>[2x]GSVYLRYFKGLILSDAYAPGLKWSDELKAYSALAFKYRDVRKYFLEKEIEVEENVIDSLPFPLIKDKIELRDYQAEAVKAWLKEKRGIIVLPTGAGKTQVALKIVSIMKVATLIVVPTIDLITQWKERINKYLDFDPGIIGGGEDSLKGITVITYDSAYTRAEELGNKFPLLIFDEVHHLPSEGYSIMAQLFASPYRLGLTATPERDDGKHELYPILVGPIVYRKSVEELAGKYIAKYKIKKLYVSLTNEEKKRYDGLRKKLKDFLSSRGLKLQNLDDFHRLVKLAAKDKEAREALLAWHESLNIAVNSQSKIEKLREILQEYKNEKIIVFTRDTQMAYRISKTFLIPVVTYKTDKDEREEILQKFRDGEYRVIVASTVFDEGVDVPDATLAIVMGGYGTKRQFLQRLGRILRKKDKEALLIEIVTKGTADYRLSR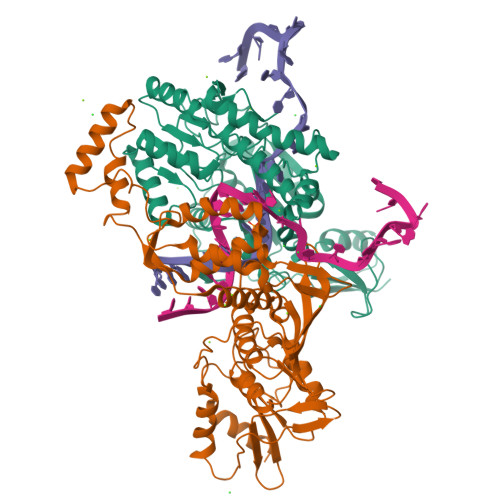RRRE;>MGLPWELARFSIVKDEVLPHFATNEDLDLANEIISLFKAGKKLGEIDEEIEYLEKIYDHKLVRAFVKLLTRLCEFELDSPIPPIQIRRELFKYGPVLDEKEREDIIQKVSKKLGADIMRFVFSDLDEEKKIIKAPTISAEDLIRWYNLSLLQTLLFKAYKLTVYVSSNWKEIIRRAKWLGLMYFAYDKPLRFEFLGPATLVKLTEKYGRNLAVLLQFIISSQNWKIEAELVLGKKFKRVYKLKLANFKELKELVIDEKRFDSSVEEKFYKDFTNVIKGWKIIREPEPLVVDNRVFIPDFLVEKGNLKVYVEIVGFWTKEYIKEKLDKLKKVKYPILILLNEELGKEKFNGMNVITYKRKIDISLVYKWLRELE[2x]> KVTMNDFDYLKLLGKGTFGKVILVREKATGRYYAMKILRKEVIIAKDEVAHTVTESRVLQNTRHPFLTALKYAFQTHDRLCFVMEYANGGELFFHLSRERVFTEERARFYGAEIVSALEYLHSRDVVYRDIKLENLMLDKDGHIKITDFGLCKEGISDGATMKTFCGTPEYLAPEVLEDNDYGRAVDWWGLGVVMYEMMCGRLPFYNQDHERLFELILMEEIRFPRTLSPEAKSLLAGLLKKDPKQRLGGGPSDAKEVMEHRFFLSINWQDVVQKKLLPPFKPQVTS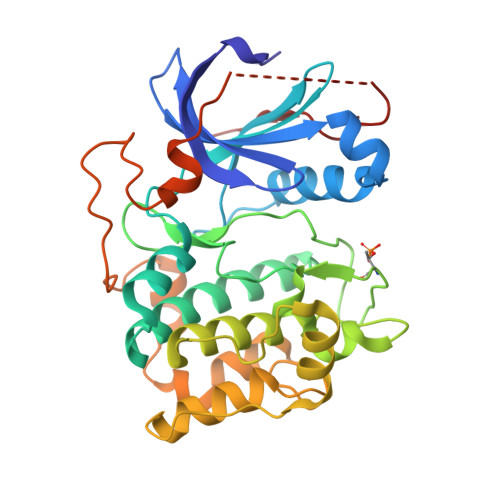EVDTRYFDDEFTAQSITITPPDRYDSLGLLELDQREEQEMFEDFDYIADW>[4x]GMKLETIDYRAADSAKRFVESLRETGFGVLSNHPIDKELVERIYTEWQAFFNSEAKNEFMFNRETHDGFFPASISETAKGHTVKDIKEYYHVYPWGRIPDSLRANILAYYEKANTLASELLEWIETYSPDEI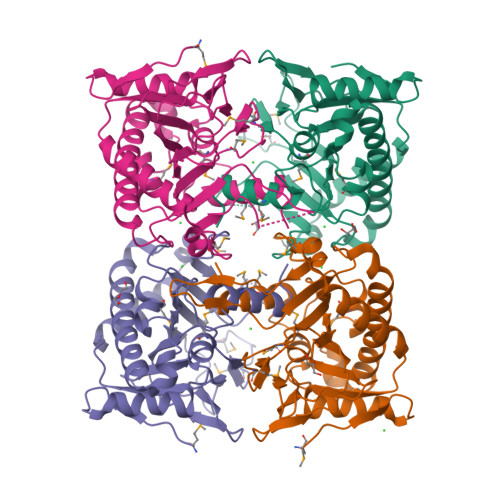KAKFSIPLPEMIANSHKTLLRILHYPPMTGDEEMGAIRAAAHEDINLITVLPTANEPGLQVKAKDGSWLDVPSDFGNIIINIGDMLQEASDGYFPSTSHRVINPEGTDKTKSRISLPLFLHPHPSVVLSERYTADSYLMERLRELGVL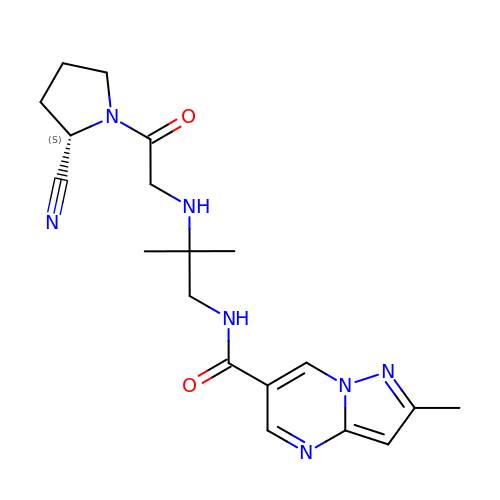N-[2-({2-[(2S)-2-cyanopyrrolidin-1-yl]-2-oxoethyl}amino)-2-methylpropyl]-2-methylpyrazolo[1,5-a]pyrimidine-6-carboxamide | C19 H25 N7 O2 | LDXYBEHACFJIEL-HNNXBMFYSA-N> MEAQPQVISATGVVKGIDLESKKITIHHDPIAAVNWPEMTMRFTITPQTKMSEIKTGDKVAFNFVQQGNLSLLQDIKVS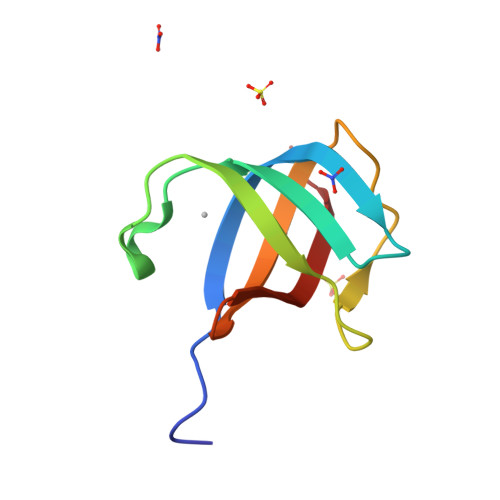Q>[2x]MQKDALNNVHITDEQVLMTPEQLKAAFPLSLQQEAQIADSRKSISDIIAGRDPRLLVVCGPCSIHDPETALEYARRFKALAAEVSDSLYLVMRVYFEKPRTTVGWKGLINDPHMDGSFDVEAGLQIARKLLLELVNMGLPLATEALDPNSPQYLGDLFSWSAIGARTTESQTH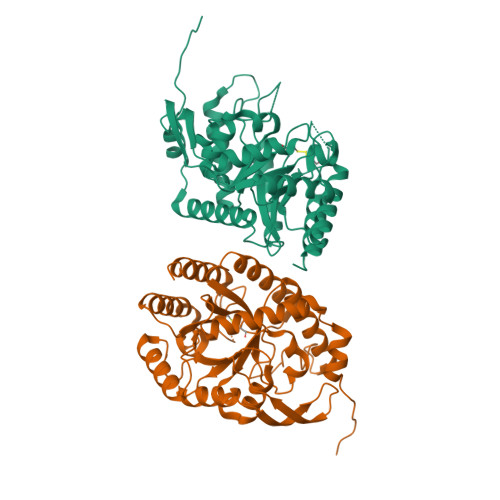REMASGLSMPVGFKNGTDGSLATAINAMRAAAQPHRFVGINQAGQVALLQTQGNPDGHVILRGGKAPNYSPADVAQCEKEMEQAGLRPSLMVDCSHGNSNKDYRRQPAVAESVVAQIKDGNRSIIGLMIESNIHEGNQSSEQPRSEMKYGVSVTDACISWEMTDALLREIHQDLNGQLTARVA>MKYMITSKGDEKSDLLRLNMIAGFGEYDMEYDDVEPEIVISIGGDGTFLSAFHQYEERLDEIAFIGIHTGHLGFYADWRPAEADKLVKLLAKGEYQKVSYPLLKTTVKYGIGKKEATYLALNESTVKSSGGPFVVDVVINDIHFERFRGDGLCMSTPSGTTAYNKSLGGALMHPSIEAMQLTEMAS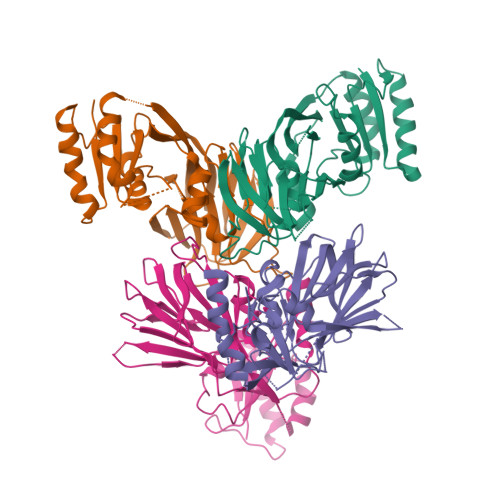INNRVYRTIGSPLVFPKHHVVSLQPVNDKDFQISVDHLSILHRDVQEIRYEVSAKKIHFARFRSFDFWRRVHDSFIEDLEHHHHHH[4x]>GSNNVPKNASALLRMNFVKGNQVLSGTGSATFIAPNVLLTVAHNFINNSADNSTGEFIGDKSKNTYEWQTPDGQKGSFTSEDIHFYNKKDYPKGFIYDLAVITLPQSTRRQHANLVENYSKVNVNDKLNVYGYPRGEYA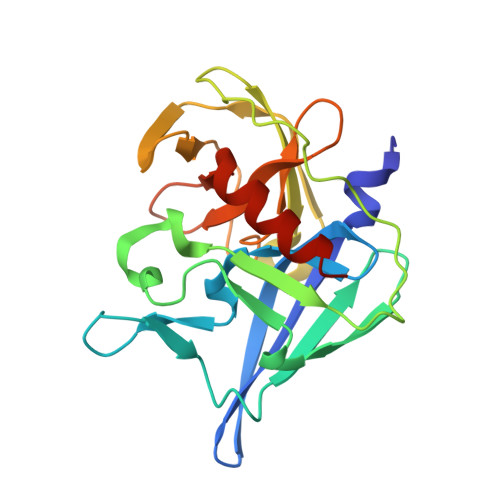HLKDTTVEIEQKYANNTYGVQYQGGKAGMSGGGIFNSKGEVIGLHQNGAENRSGGLILSPTQLDWIRSIIKGKEIT[2x]>NNDMKLAPPTDVRSGYIRLVKNVNYYIDSESIWVDNQEPQIVHFDAVVNLDKGLYVYPEPKRYARSVRQYKILNCANYHLTQVRTDFYDEFWGQGLRAAPKKQKKHTLSLTPDTTLYNAAQIICANY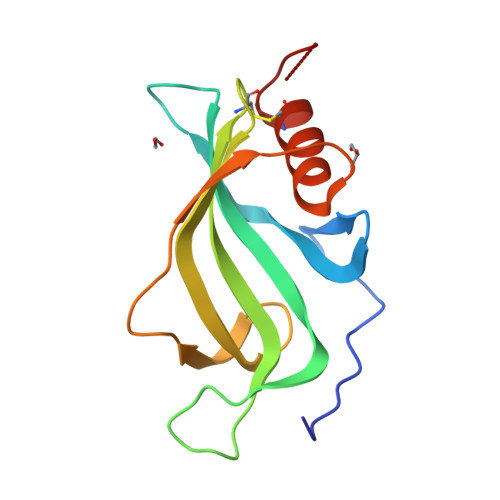GKAFSVD[2x]> SNANNLPSPSRNKYQNARRVLNSAETQNLPGRESQLQELREFFSNHLESQTSGSLYVSGQPGTGKTACLSLLLRDPDFSKRLQRVYINCTSIASVGAVYKKLCTELQLKVSGRTERDHLEAIQRHLKTAKRMLLLVLDEIDQLCTSRQEVLYTIFEWPALPGSRILLVGIANSLDLTDRALMRLNARCELKPRLMHFPPYSKQQIVEIFKSRLAEAEVLDVFPPVTLQLLAAKVSAISGDVRRALDIGRRVVEIAEQQKRDGEKEFNMKALQLEGKDAVEAKEKQDTLKPVQVTQVAAVLNKVYGASQNLEEDIEASFPLQQKLMLCTLVLMLRNERNKDISMGRLHEVYRRVCAKRNILALDQAEFTGTV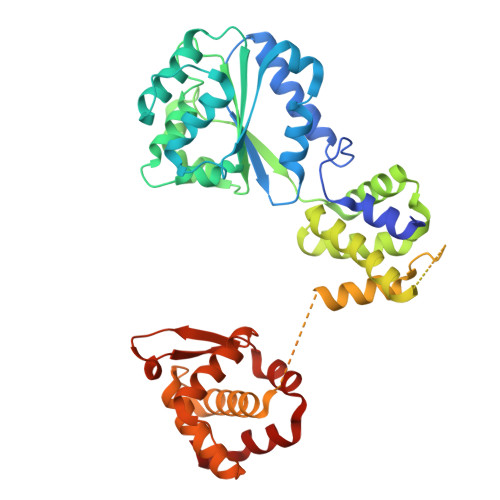DLVETRGILRIMRKKEPRLHKVLLQWDEEEVHAALSDKQLIASILSDTACLSK> MEGMRRPTPTVYVGRVPIGGAHPIAVQSMTNTPTRDVEATTAQVLELHRAGSEIVRLTVNDEEAAKAVPEIKRRLLAEGAEVPLVGDFHFNGHLLLRKYPKMAEALDKFRINPGTLGRGRHKDEHFAEMIRIAMDLGKPVRIGANWGSLDPALLTELMDRNARRPEPKSAHEVVLEALVESAVRAYEAALEMGLGEDKLVLSAKVSKARDLVWVYRELARRTQAPLHLGLTEAGMGVKGIVASAAALA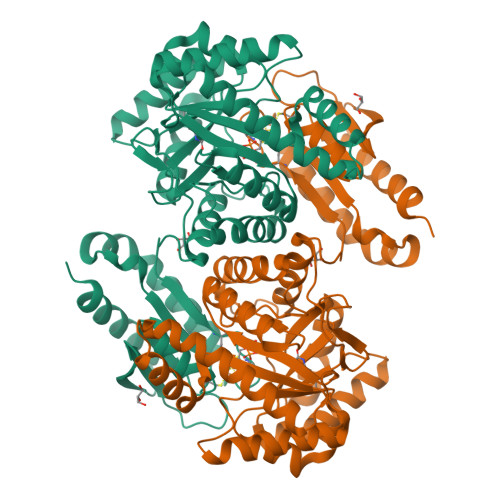PLLLEGIGDTIRVSLTPAPGEPRTKEVEVAQEILQALGLRAFAPEVTSCPGCGRTTSTFFQELAEEVSRRLKERLPEWRARYPGVEELKVAVMGCVVNGPGESKHAHIGISLPGAGEEPKAPVYADGKLLTILKGEGIAEEFLRLVEDYVKTRFAPKA> SSLDDKPQFPGASAEFIDKLEFIQPNVISGIPIYRVMDRQGQIINPSEDPHLPKEKVLKLYKSMTLLNTMDRILYESQRQGRISFYMTNYGEEGTHVGSAAALDNTDLVFGAYREAGVLMYRDYPLELFMAQCYGNISDLGKGRQMPVHYGCKERHFVTISSPLATQIPQAVGAAYAAKRANANRVVICYFGEGAASEGDAHAGFNFAATLECPIIFFCRNNGYAISTPTSEQYRGDGIAARGPGYGIMSIRVDGNDVFAVYNATKEARRRAVAENQPFLIEAMTYRIGHASTS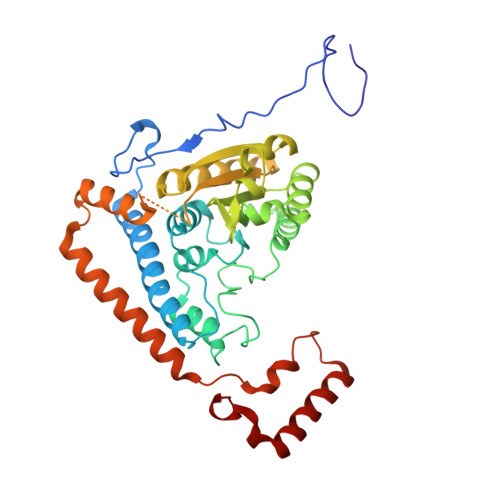DDSSAFRSVDEVNYWDKQDHPISRLRHYLLSQGWWDEEQEKAWRKQSRRKVMEAFEQAERKPKPNPNLLFSDVYQEMPAQLRKQQESLARHLQTYGEHYPLDHFDK>SEISRQEFQRRRQALVEQMQPGSAALIFAAPEVTRSADSEYPYRQNSDFWYFTGFNEPEAVLVLIKSDDTHNHSVLFNRVRDLTAEIWFGRRLGQDAAPEKLGVDRALAFSEINQQLYQLLNGLDVVYHAQGEYAYADVIVNSALEKLRKGSRQNLTAPATMIDWRPVVHEMRLFKSPEEIAVLRRAGEITAMAHTRAMEKCRPGMFEYHLEGEIHHEFNRHGARYPSYNTIVGSGENGCILHYTENECEMRDGDLVLIDAGCEYKGYAGDITRTFPVNG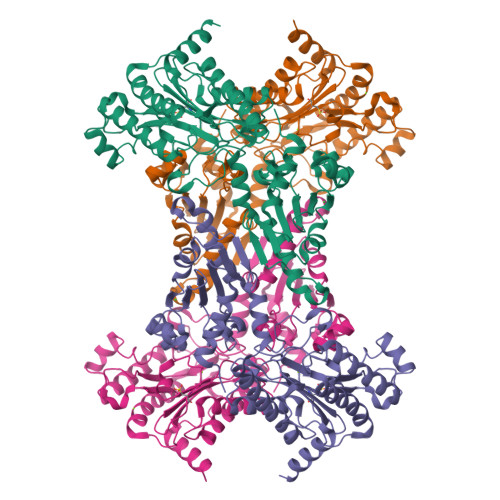KFTQAQREIYDIVLESLETSLRLYRPGTSILEVTGEVVRIMVSGLVKLGILKGDVDELIAQNAHRPFFMHGLSHWLGLDVHDVGVYGQDRSRILEPGMVLTVEPGLYIAPDAEVPEQYRGIGIRIEDDIVITETGNENLTASVVKKPEEIEALMVAARKQ[4x]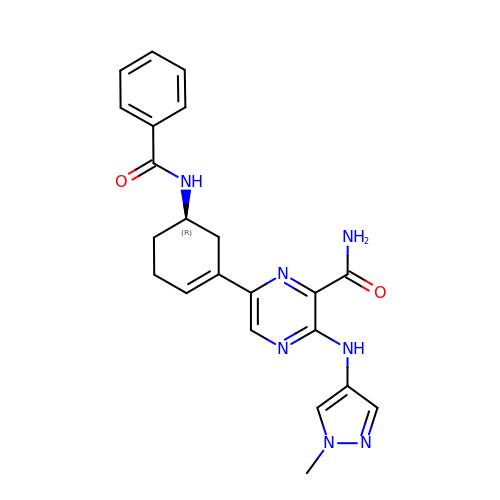6-[(5R)-5-benzamidocyclohex-1-en-1-yl]-3-[(1-methyl-1H-pyrazol-4-yl)amino]pyrazine-2-carboxamide | C22 H23 N7 O2 | HGABYPLXBWLABT-MRXNPFEDSA-N> SERCDDWGLDTMRQIQVFEDEPARIKCPLFEHFLKYNYSTAHSSGLTLIWYWTRQDRDLEEPINFRLPENRISKEKDVLWFRPTLLNDTGNYTCMLRNTTYCSKVAFPLEVVQKDSCFNSAMRFPVHKMYIEHGIHKIT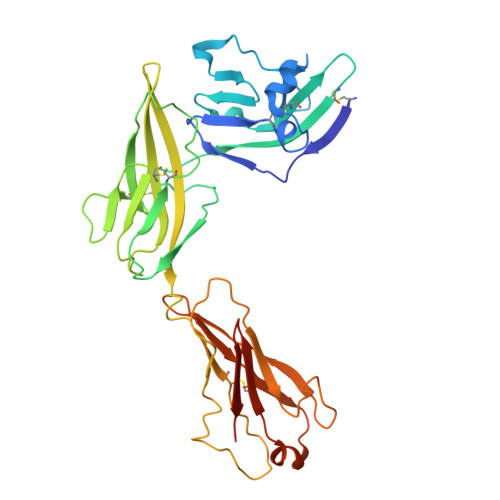CPNVDGYFPSSVKPSVTWYKGCTEIVDFHNVLPEGMNLSFFIPLVSNNGNYTCVVTYPENGRLFHLTRTVTVKVVGSPKDALPPQIYSPNDRVVYEKEPGEELVIPCKVYFSFIMDSHNEVWWTIDGKKPDDVTVDITINESVSYSSTEDETRTQILSIKKVTPEDLRRNYVCHARNTKGEAEQAAKVKQKVAAHHHHHH> MGSDKIHHHH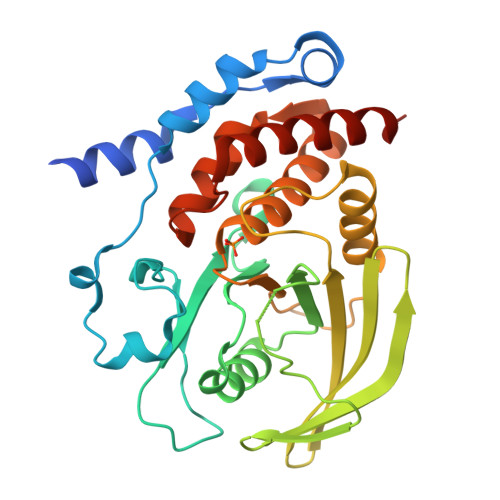HHMNTPREVTLHFLRTAGHPLTRWALQRQPPSPKQLEEEFLKIPSNFVSPEDLDIPGHASKDRYKTILPNPQSRVCLGRAQSQEDGDYINANYIRGYDGKEKVYIATQGPMPNTVSDFWEMVWQEEVSLIVMLTQLREGKEKCVHYWPTEEETYGPFQIRIQDMKECPEYTVRQLTIQYQEERRSVKHILFSAWPDHQTPESAGPLLRLVAEVEESPETAAHPGPIVVHCSAGIGRTGCFIATRIGCQQLKARGEVDILGIVCQLRLDRGGMIQTAEQYQFLHHTLALYAGQLPEEPSP> APKCIECHINIEMDPVLHDVFKLQVCKQCSKEHPEKYALLTKTECKEDYFLTDPELNDEDLFHRLEKPNPHSGTFARMQLFVRCEVEAFAFKKWGGEEGLDEEWQRREEGKAHRREKKY;> MTPEQKAKLEANRKLAIERLRKRGILSSDQLNRIESRNEPLKTRPLAVTSGSNRDDNAAAAVHVPNHNGQPSALANTNTNTTSLYGSGVVDGSKRDASVLDKRPTDRIRPSIRKQDYIEYDFATMQNLNGGYINPKDKLPNSDFTDDQEFESEFGSKKQKTLQDWKKEQLERKMLYENAPPPEHISKAPKCIECHINIEMDPVLHDVFKLQVCKQCSKEHPEKYALLTKTECKEDYFLTDPELNDEDLFHRLEKPNPHSGTFARMQLFVRCEVEAFAFKKWGGEEGLDEEWQRREEGKAHRREKKYEKKIKEMRLKTRAQEY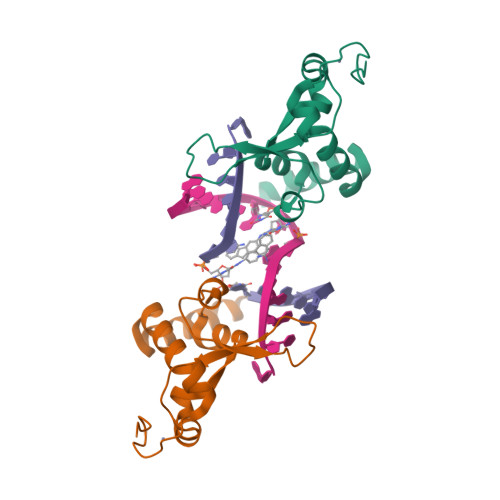TNRLREKKHGKAHIHHFSDPVDGGIDEDGYQIQRRRCTDCGLETEEIDI>TRDQNGTWEMESNENFEGYMKALDIDFCTRKIAVRCTQTKVI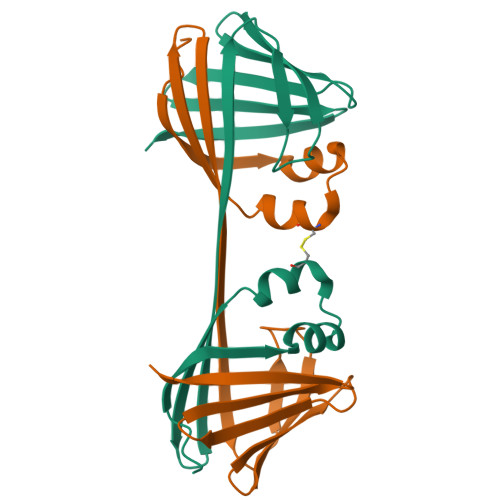DQDGDNFKDKTTSTFHHHRNYDVDFTVGVEFDEYTKSLDNRHVKALVTWEGDVLVCVQKGEKENRGWKKWIEGDKLYLELTCGDQVCRQVFKKK[2x]Angiogenin, also referred to as RNase 5, is a small 123-amino-acid protein and a member of the bovine pancreatic ribo­nuclease A (RNase A) superfamily. Although it has been assigned various regulatory roles, its core catalytic function is that of an RNA endonuclease. Angiogenin from humans shares a high degree of sequence similarity with the eponymous member of the superfamily, and the catalytic triad consisting of a lysine (Lys40) and two histidines (His13 and His114) is conserved between the two enzymes. However, angiogenin features a unique C-terminal 310-helix and its B2 site is occluded by Gln117, which is locked in place through a hydrogen bond to Thr44.

Here, we present the crystal structure of two angiogenin molecules bound to an RNA duplex in a dimer-like fashion. A complex of the inactive angiogenin variant H114A and a 19-mer RNA was prepared by mixing and incubation on ice. The unit cell contains two molecules of angiogenin (chains A and B) and one double-stranded RNA duplex (chains C and D). Since the RNA sequence was not designed to be self-complementary, the RNA complex, made up of two strands of identical sequence, contains three mismatches. All of these interactions are sequence-independent backbone contacts. Another RNA contact is mainly mediated by the angiogenin-specific C-terminal helix 4, which is located close to the active site. In both angiogenin chains this helix contributes Arg121 and Arg122, which interact with opposite strands across the minor groove. Here, the helix remains in an identical position in both chains and the RNA binding that is observed in this structure does not trigger a structural rearrangement.

>QDNSRYTHFLTQHYDAKPQGRDDRYCESIMRRRGLTSPCKDINTFIHGNKRSIKAICENKNGNPHRENLRISKSSFQVTTCKLHGGSPWPPCQYRATAGFRNVVVACENGLPVALDQSIFRRP[2x]[(2~{S},3~{S},4~{S},5~{R},6~{S})-6-octoxy-3,4,5-tris(oxidanyl)oxan-2-yl]methanesulfonic 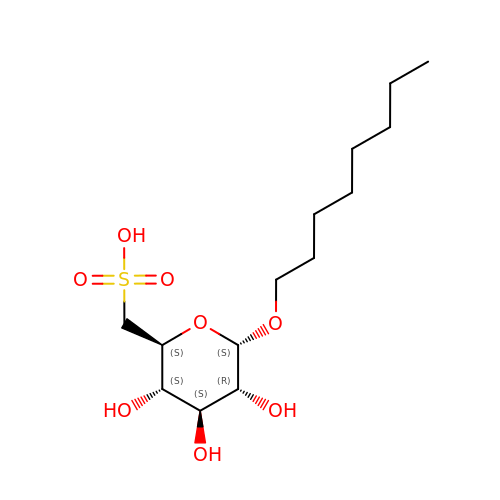acid | C14 H28 O8 S | MGTVINCFAITWEK-RGDJUOJXSA-N> GLGGLERFCSPGKGRGLRALQPFQVGDLLFSCPAYAYVLTVNERGNHCEYCFTRKEGLSKCGRCKQAFYCNVECQKEDWPMHKLECSPMVVFGENWNPSETVRLTARILAKQKIHPERTPSEKLLAVKEFESHLDKLDNEKKDLIQSDIAALHHFYSKHLEFPDN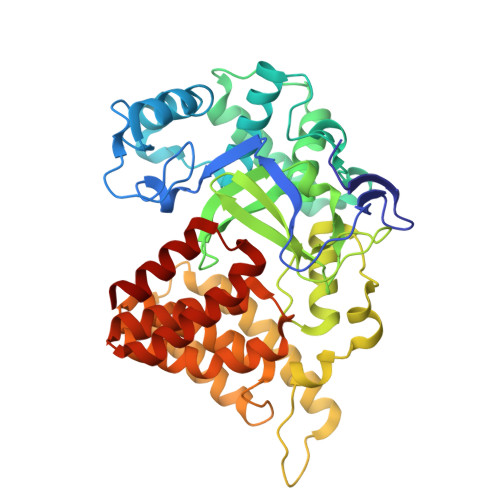DSLVVLFAQVNCNGFTIEDEELSHLGSAIFPDVALMNHSCCPNVIVTYKGTLAEVRAVQEIKPGEEVFTSYIDLLYPTEDRNDRLRDSYFFTCECQECTTKDKDKAKVEIRKLSDPPKAEAIRDMVRYARNVIEEFRRAKHYKSPSELLEICELSQEKMSSVFEDSNVYMLHMMYQAMGVCLYMQDWEGALQYGQKIIKPYSKHYPLYSLNVASMWLKLGRLYMGLEHKAAGEKALKKAIAIMEVAHGKDHPYISEIKQEIESH>[2x]GGGCUUCGUUAGGUGAGGCUCCUGUAUGGAGAUACGCUGCUGCCCAAAAAUGUCCAAAGACGCCAAUGGGUCAACAGAAAUCAUCGACAUAAGGU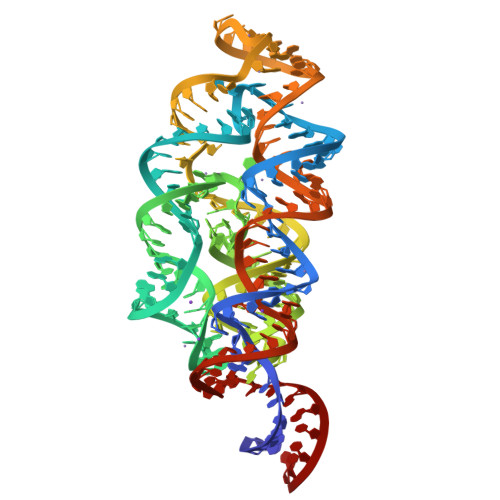GAUUUUUAAUGCAGCUGGAUGCUUGUCCUAUGCCAUACAGUGCUAAAGCUCUACGAUUGAAGCCCA> MSYNFPAVNQLKSSKDIPDPFIFMDGSKVESTDDWWKRQSEISCMYEYYMYGKWIDGSDDETTYSISGNSMTINVKRKSTGKTASFKAVINLPKNVRHEGGAPVILGMHKGISESTATSNGYAVITYDSDGMFSAPGTAQDNNQHKGAFYDLYPYGRNWDEQTGDLMAWSWGISRILDALYNGAAKELNINPDSSIVTGVSRYGKA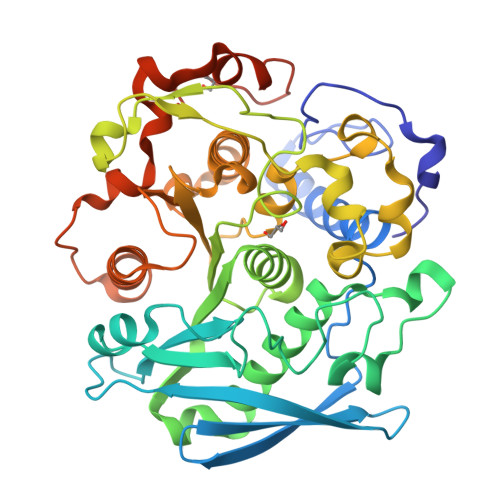ASVCGAFDTRIKMCAPSCSGAGGLALYRYSSVGKTYDFSSKGGSSSYTYKENEPLGSLQASGEQGWFNGRFMEFRNAEQFPMDQHMLGALCCDPDRYLFIIGSCESEDWVNAPSVWMAYLGMKHVWDYVGISDHLAINIHKSGHAVIAEDIEKMVQYFDYHVYGIQPKMNLEELQTSVFALPKNKDSFADTFASKWLYDPAFLYKVPAFLYKVVIMHHHHHH The recent identification of SmbA, an effector protein from Caulobacter crescentus that is jointly targeted by both signaling molecules, has opened up studies on how these global bacterial networks interact. C-di-GMP and (p)ppGpp compete for the same SmbA binding site, with a dimer of c-di-GMP inducing a conformational change that involves loop 7 of the protein that leads to downstream signaling. SmbA stimulates Caulobacter growth on glucose while preventing surface attachment in its active state repressed by binding of the c-di-GMP dimer. The major conformational changes promoting SmbA’s functional switch affect the C-terminal helix 9 and the flexible loop 7 containing c-di-GMP subsite residues R211 and D214 from the RxxD motif.

To understand how a flexible loop 7 influences the overall SmbA structure and its ligand binding, we present here the high-resolution structure of a loop 7 deletion mutant (fragment 198–215, hereafter SmbA∆loop). In addition to the SmbA∆loop/c-di-GMP complex, we also determined a crystal structure of the protein in the absence of c-di-GMP. The Crystal contains four molecules in the asymmetric unit. Overall, apo SmbA∆loop shows virtually the same structure as in complex with c-di-GMP with an rmsd value of 0.49 Å for 225 Cα atoms. Overall, the SmbA∆loop mutant retains the TIM-barrel fold with eight α-helices on the outside and eight parallel β-strands on the inside with an extra helix 9. Importantly, in the SmbA∆loop mutant, C-terminal helix 9 adopts an outward orientation similar to that found in the ppGpp-bound active state of the protein. As measured directly by sedimentation velocity analytical ultracentrifugation (AUC-SV), apo SmbA∆loop is monomeric with a sedimentation coefficient of 1.73 s. For completeness, the affinity of ppGpp to the SmbA mutant was also measured and was found to be virtually identical to the affinity of the compound to SmbAw31t indicating that loop 7, as expected, does not contribute to ppGpp binding.

>MRYRPFGSTGVAVSALTLRLADNPRLRANDWRALVFTALENGVNSFQIDGDAPELLKGAGEAFASVERHLLFLTWRLRGDAKQLGPHTLDALKRSAFEGLSLDYLDLLLINDPQSASLPMAFESGLQDLQKGRALRGLGVASRGDIDPGLLANDLVTAVSSPYNLSSGWAERHRIRQASQNNFAVIGEDFWPQALRELADVGGYEFLTNTPGWSAEDICLGYALTEPSLATVRVTADNRQEIERLAAVVERDLPTGVCAQIEMARFSAQEREKAARRPKLAAALEHHHHEK[4x]> MAHHHHHHKVRLDPSRCVGHAQCYAVDPDLFPIDDSGNSILAEHEVRPEDMQLTRDGVAACPEMALILEEDDADVLHRHQPVTIGEPAAKKTTTPGEDHAGSFYLPRLEYSTLPMAVDRGVGWKTLRDAGPVVFMNGWYYLTRREDVLAALRNPKVFSSRKALQPPGNPLPVVPLAFDPPEHTRYRRILQPYFSPAALSKALPSLRRHTVAMIDAIAGRGECEAMADLANLFPFQLFLVLYGLPLEDRDRLIGWKDAVIAMSDRPHPTEADVAAARELLEYLTAMVAERRRNPGPDVLSQVQIGEDPLSEIEVLGLSHLLILAGLDTVTAAVGFSLLELARRPQLRAMLRDNPKQIRVFIEEIV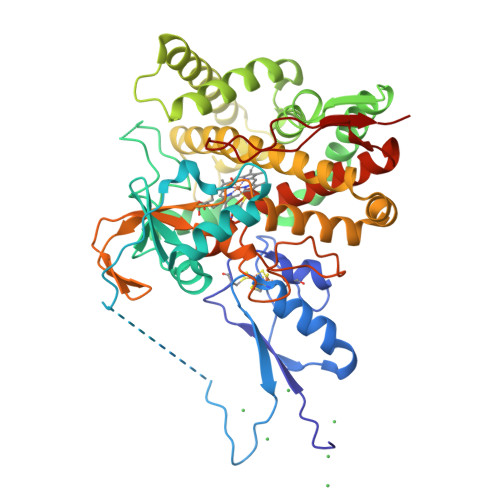RLEPSAPVAPRVTTEPVTVGGMTLPAGSPVRLCMAAVNRDGSDAMSTDELVMDGKVHRHWGFGGGPHRCLGSHLARLELTLLVGEWLNQIPDFELAPDYAPEIRFPSKSFALKNLPLRWS>[4x]MVQEIDLGLTCDMHVHVREGAMCELVTPKIRDGGVSIAYIMPNLQPPITTLDRVIEYKKTLQKLAPKT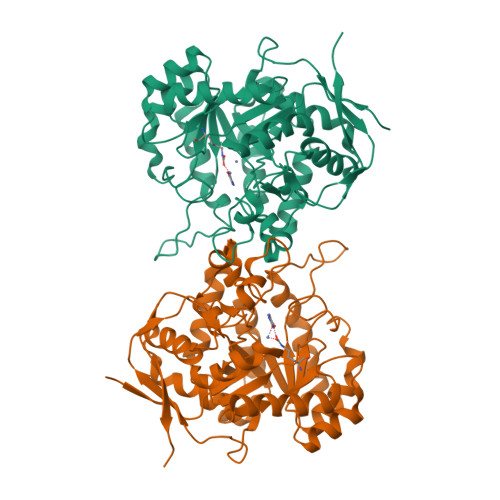TFLMSFYLSKDLTPDLIHEAAQQHAIRGVKCYPAGVTTNSAAGVDPNDFSAFYPIFKAMQEENLVLNLHGEKPSVHDGDKEPIHVLNAEEAFLPALKKLHNDFPNLKIILEHCTSESAIKTIEDINKNVKKATDVKVAATLTAHHLFLTIDDWAGNPVNFCKPVAKLPNDKKALVKAAVSGKPYFFFGSDSAPHPVQNKANYEGVCAGVYSQSFAIPYIAQVFEEQNALENLKGFVSDFGISFYEVKDSEVASSDKAILFKKEQVIPQVISDGKDISIIPFKAGDKLSWSVRWEPRLEHHHHHH> GSIYT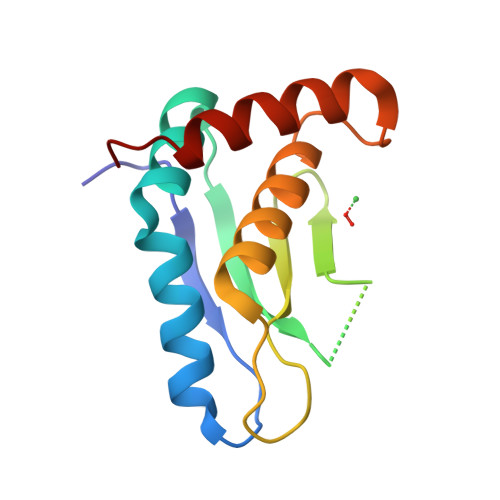FNELVVLDYPHKDRALRYLERLRDDTGIKKIMDSHRWTVPLLSEMDPAEHTRHDSKTLGLNHNQGAHIELRLRTDRYDGFRDYKTVKSTLIHELTHNVHGEHDSSFWELFRQLTKEADAADL> YDDGICKSSDCIKSAARLIQNMDATTEPCTDFFKYACGGWLKRNVIPETSSRYGNFDILRDELEVVLKDVLQEPKTEDIVAVQKAKALYRSCINESAIDSRGGEPLLKLLPDIYGWPVATENWEQKYGASWTAEKAIAQLNSKYGKKVLINLFVGTDDKNSVNHVIHIDQPRLGLPSRDYYECTGIYKEACTAYVDFMISVARLIRQEERLPIDENQLALEMNKVMELEKEIANATAKPEDRNDPMLLYNKMTLAQIQNNFSLEINGKPFSWLNFTNEIMSTVNISITNEEDVVVYAPEYLTKLKPILTKYSARDLQNLMSWRFIMDLVSSLSRTYKESRNAFRKALYGTTSETATWRRCANYVNGNMENAVGRLYVEAAFAGESKHVVEDLIAQIREVFIQTLDDLTWMDAETKKRAEEKALAIKERIGYPDDIVSNDNKLNNEYLELNYKEDEYFENIIQNLKFSQSKQLKKLREKVDKDEWISGAAVVNAFYSSGRNQIVFPAGILQPPFFSAQQSNSLNYGGIGMVIGHEIT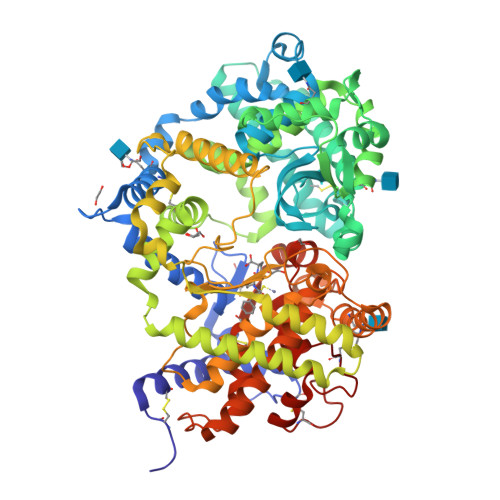HGFDDNGRNFNKDGDLVDWWTQQSASNFKEQSQCMVYQYGNFSWDLAGGQHLNGINTLGENIADNGGLGQAYRAYQNYIKKNGEEKLLPGLDLNHKQLFFLNFAQVWCGTYRPEYAVNSIKTDVHSPGNFRIIGTLQNSAEFSEAFHCRKNSYMNPEKKCRVW>[2x]GSTDIEDLDLYATSRERRFRLFASIECEGQLFMTPYDFILAVTTDEPKVAKTWKSLSKQELNQMLAETPPVWKGSSKLFRNLKEKGVISYTEYLFLLCILTKPHAGFRIAFNMFDTDGNEMVDKKEFLVLQEIFRKKNEKREIKGDEEKRAMLRLQLYGYHSPTNSVLKTDAEELVSRSYWDTLRRNTSQALFSDL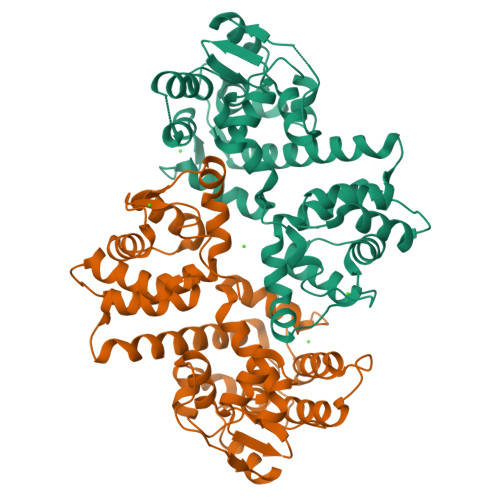AERADDITSLVTDTTLLVHFFGKKGKAELNFEDFYRFMDNLQTEVLEIEFLSYSNGMNTISEEDFAHILLRYTNVENTSVFLENVRYSIPEEKGITFDEFRSFFQFLNNLEDFAIALNMYNFASRSIGQDEFKRAVYVATGLKFSPHLVNTVFKIFDVDKDDQLSYKEFIGIMKDRLHRGFRGYKT>[2x]MSFTPANRAYPYTRLRRNRRDDFSRRLVRENVLTVDDLILPVFVLDGVNQRESIPSMPGVERLSIDQLLI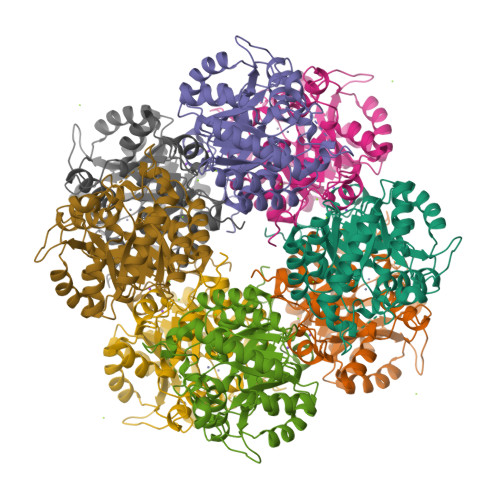EAEEWVALGIPALALFPVTPVEKKSLDAAEAYNPEGIAQRATRALRERFPELGIITDVCLCEFTTHGQCGILDDDGYVLNDVSIDVLVRQALSHAEAGAQVVAPSDMMDGRIGAIREALESAGHTNVRVMAYSAKYASAYYGPFRDAVGSASNLGKGNRATYQMDPANSDEALHEVAADLAEGADMVMVKPGMPYLDIVRRVKDEFRAPTFVYQVSGEYAMHMGAIQNGWLAESVILESLTAFKRAGADGILTYFAKQAAEQLRRGR Promyelocytic leukemia protein (PML), belonging to the TRIM family, serves as a valuable model in this field. Within the nucleus, this 70 kDa PML protein molecule has the capability to assemble into a super protein complex, known as PML nuclear bodies (NBs). PML NBs participate in various important cellular pathways, including DNA damage repair, transcriptional regulation, self-renewal of stem cells, regulation of p53 stability, cell proliferation, apoptosis, and defense against viral infections. The RING and B-box domains are zinc-binding domains.

In this study, we report the cryo-EM structure of the PML46–256 dimer, which encompasses the entire RING-B1-B2 domains and a segment of the CC domain. After multiple rounds of 2D and 3D classification to eliminate heterogeneous and incomplete components, we determined the cryo-EM structure of PML46–256 at an overall resolution of 5.3 Å, with the core region slightly better resolved (~4.4 Å). In our cryo-EM model, each PML monomer comprises helices α1–α7 and beta strands β1–β7. Unlike other TRIMs, the RING, B1 and B2 subdomains are folded together, centered around the PML α3 helix, resulting in a PML monomer. The RING, B1, and B2 domains are arranged surrounding the α3 helix and are distributed on the outer surface of the PML molecule. In this inner α3 helix, residues F108, F109, L112, and L116 form a hydrophobic core, intermittently mediating the engagement of the PML RING, B1 and B2, respectively. The current cryo-EM structure revealed that the PML monomer, which serves as the basic unit for assembling PML NBs, forms a functional PML dimer via two α6 helices. Specifically, V123, F177, and L178 within the α6 helix from one monomer interact with their counterparts from the other monomer, facilitating this dimerization. Additionally, two SUMOylation sites, K65 and K160, are located on the outer surface of the dimeric PML46–256, giving ample space for PML SUMOylation. Despite the prediction that the CC domain would be a long helix, the density of the C-terminal CC residues 236–256 were not visible in this PML dimer. Furthermore, based on the current model, the C-terminal S221 residues from the two monomers locate on opposite sides of the PML dimer, facing away from the dimeric interface. This suggests that the two PML CC helices following S221 might be positioned on opposite sides of the PML dimer, resembling the arms of an octopus.

>PASEEEFQFLRCQQCQAEAKCPKLLPCLHTLCSGCLEASGMQCPICQAPWPLGADTPALDNVFFESLQRRLSVYRQIVDAQAVCTRCKESADFWCFECEQLLCAKCFEAHQWFLKHEARPLAELRNQSVREFLDGTRKTNNIFCSNPNHRTPTLTSIYCRGCSKPLCCSCALLDSSHSELKCDISAEIQQRQEELDAMTQALQEQDSAFGA[2x]> YFGKLESKLSVIRNLNDQVLFIDQGNRPLFEDMTDS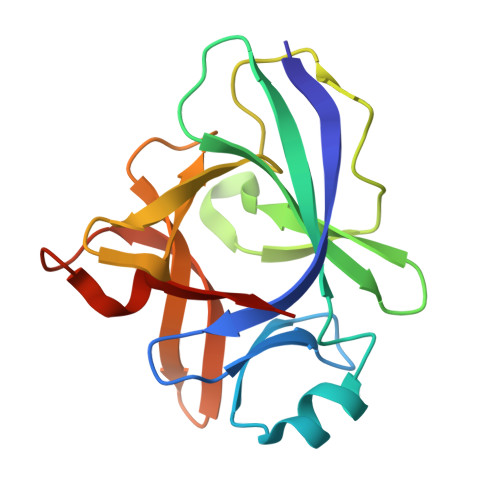DSRDNAPRTIFIISMYKDSQPRGMAVTISVKSEKISTLSSENKIISFKEMNPPDNIKDTKSDIIFFQRSVPGHDNKMQFESSSYEGYFLASEKERDLFKLILKKEDELGDRSIMFTVQNED>[2x]AALGVQSINWQTAFNRQAHHTDKFSSQELILRRGQNFQVLMIMNKGLGSNERLEFIVSTGPYPSESAMTKAVFPLSNGSSGGWSAVLQASNGNTLTISISSPASAPIGRYTMALQIFSQGGISSVKLGTFILLFNPWLNVDSVFMGNHAEREEYVQEDAGIIFVGSTNRIGMIGWNFGQFEEDILSICLSILDRSLNFRRDAATDVASRNDPKYVGRVLSAMINSNDDNGVLAGNWSGTYTGGRDPRSWDGSVEILKNWKKS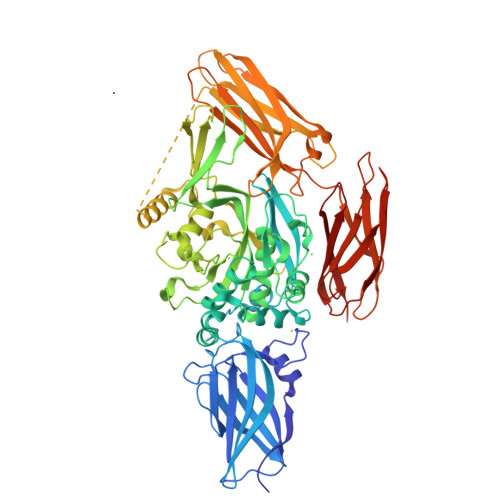GLSPVRYGQCWVFAGTLNTALRSLGIPSRVITNFNSAHDTDRNLSVDVYYDPMGNPLDKGSDSVWNFHVWNEGWFVRSDLGPSYGGWQVLDATPQERSQGVFQCGPASVIGVREGDVQLNFDMPFIFAEVNADRITWLYDNTTGKQWKNSVNSHTIGRYISTKAVGSNARMDVTDKYKYPEGSDQERQVFQKALGKLKPNTPFAATSSMGLETEEQEPSIIGKLKVAGMLAVGKEVNLVLLLKNLSRDTKTVTVNMTAWTIIYNGTLVHEVWKDSATMSLDPEEEAEHPIKISYAQYERYLKSDNMIRITAVCKVPDESEVVVERDIILDNPTLTLEVLNEARVRKPVNVQMLFSNPLDEPVRDCVLMVEGSGLLLGNLKIDVPTLGPKERSRVRFDILPSRSGTKQLLADFSCNKFPAIKAMLSIDVAE>SPLHFAASYGRINTCQRLLQDISDTRLLNEGDLHGMTPLHLAAKNGHDKVVQLLLKKGALFLSDHNGWTALHHASMGGYTQTMKVILDTNLKCTDRLDEDGNTALHFAAREGHAKAVALLLSHNADIVLNKQQASFLHLALHNKRKEVVLTIIRSKRWDECLKIFSHNSPGNKCPITEMIEYLPECMKVLLDFCMLHSTEDKSCRDYYIEYNFKYLQCPLEFTKKTPTQDVIYEPLTALNAMVQNNRIELLNHPVCKEYLLMKWLAYGFRAHMMNLGSYCLGLIPMTILVVNIKPGMAFNSTGIINETSDHSEILDTTNSYLIKTCMILVFLSSIFGYCKEAGQIFQQKRNYFMDISNVLEWIIYTTGIIFVLPLFVEIPA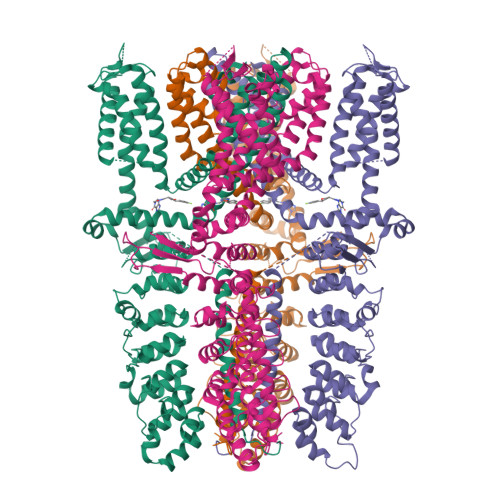HLQWQCGAIAVYFYWMNFLLYLQRFENCGIFIVMLEVILKTLLRSTVVFIFLLLAFGLSFYILLNLQDPFSSPLLSIIQTFSMMLGDINYRESFLEPYLRNELAHPVLSFAQLVSFTIFVPIVLMNLLIGLAVGDIADVQKHASLKRIAMQVELHTSLEKKLPLWFLRKVDQKSTIVYPNKPRSGGMLFHIFCFLFCTGEIRQEIPNADKSLEMEILKQKYRLKDLTFLLEKQHELIKLIIQKMEIISET[4x]>[2x]ETAGVSENAKLIVKKTFDSYTDNEVLMPKADYTFKVEADSTASGKTKD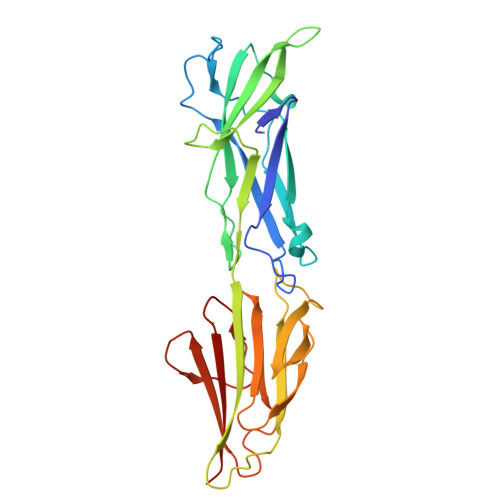GLEIKPGIVNGLTEQIISYTNTDKPDSKVKSTEFDFSKVVFPGIGVYRYIVSEKQGDVEGITYDTKKWTVDVYVGNKEGGGFEPKFIVSKEQGTDVKKPVNFNNSFATTSLKVKKNVSGNTGELQKEFDFTLTLNESTNFKKDQIVSLQKGNEKFEVKIGTPYKFKLKNGESIQLDKLPVGITYKVNEMEANKDGYKTTASLKEGDGQSKMYQLDMEQKTDESADEIVVTNKRD> ARPCIPKSFGYSSVVCVCNATYCDSFDPPTFPALGTFSRYESTRSGRRMELSMGPIQANHTGTGLLLTLQPEQKFQKVKGFGGAMTDAAALNILALSPPAQNLLLKSYFSEEGIGYNIIRVPMASCDFSIRTYTYADTPDDFQLHNFSLPEEDTKLKIPLIHRALQLAQRPVSLLASPWTSPTWLKTNGAVNGKGSLKGQPGDIYHQTWARYFVKFLDAYAEHKLQFWAVTAENEPSAGLLSGYPFQCLGFTPEHQRDFIARDLGPTLANSTHHNVRLLMLDDQRLLLPHWAKVVLTDPEAAKYVHGIAVHWYLDFLAPAKATLGETHRLFPNTMLFASEACVGSKFWEQSVRLGSWDRGMQYSHSIITNLLYHVVGWTDWNLALNPEGGPNWVRNFVDSPIIVDITKDTFYKQPMFYHLGHFSKFIPEGSQRVGLVASQKNDLDAVALMHPDGSAVVVVLNRSSKDVPLTIKDPAVGFLETISPGYSIHTYLWRRQ

The lysosomal glycoside hydrolase β-glucocerebrosidase (GBA; sometimes called GBA1 or GCase) catalyses the hydrolysis of glycosphingolipids. Mechanistically, GBA is a retaining β-glucosidase which hydrolyses its substrates with net retention of β-anomeric stereochemistry. Retention of anomeric configuration is achieved through the Koshland double-displacement mechanism using two key carboxylate-containing residues; in the case of human GBA, Glu340 serves as the catalytic nucleophile and Glu235 acts as the general acid/base. Inherited deficiencies in GBA activity cause an accumulation of GlcCer within lysosomes, subsequently leading to the most common lysosomal storage disorder, Gaucher disease (GD; Grabowski & Horowitz, 1997; Brady et al., 1966). Here, the production of active crystallizable GBA in insect cells using a baculovirus expression system is reported, providing a nonclinical source of recombinant GBA with comparable activity and biophysical properties to ERT preparations.

Consequently, our GBA was studied by X-ray crystallography to generate a 0.98 Å resolution unliganded structure in a novel crystal form. During initial screening, crystals were also found under condition A5 [0.2 M magnesium formate, 20%(w/v) PEG 3350] of the JCSG-plus screen. Optimized crystals suitable for structural analysis were obtained using 0.2 M magnesium formate, 19%(v/v) PEG 3350. Previously, GBA has been crystallized in space groups C2221 and P21; however, this unliganded structure crystallized in space group P1. Overall, the three-domain tertiary structure is highly similar to that of the BTP complex and Cerezyme, with Cα r.m.s.d.s of 0.49 Å (Q score of 0.94) and 0.60 Å (Q score of 0.94), respectively. Despite the sub-Ångström resolution, residues 26–31 and 314–319 were challenging to model, reflecting the flexibility and disorder of these loops, which has also been observed in previous GBA structures. Importantly, the active site of this unliganded structure compares well with the active sites of Cerezyme and the BTP complex. The sub-Ångström resolution of this unliganded structure permits the first ever atomic resolution analysis of GBA, uncovering finer details in its structure. In fact, many alternative side-chain conformations could be modelled throughout the structure, providing more detail on side-chain mobility and interactions. Multiple alternative residue conformations were observed throughout the structure, including two conformations of the catalytic acid/base residue.>[2x]RSQHTCSISKVTSLLEVNCENKKLTALPADLPADTGILHLGENQLGTFSTASLVHFTHLTYLYLDRCELTSLQTNGKLIKLENLDLSHNNLKSLPSLGWALPALTTLDVSFNKLGSLSPGVLDGLSQLQELYLQNNDLKSLPP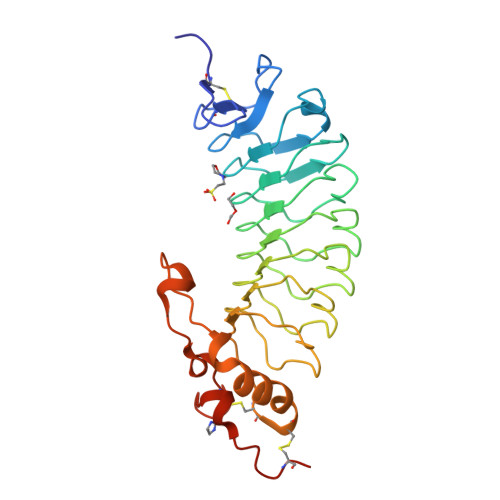GLLLPTTKLKKLNLANNKLRELPSGLLDGLEDLDTLYLQRNWLRTIPKGFFGTLLLPFVFLHANSWYCDCEILYFRHWLQENANNVYLWKQGVDVKDTTPNVASVRCANLDNAPVYSYPGKGCPTTRTGHHHHHH>[2x]MLIKPKRLQAGDIVATVSPSWGGAGDSEIRWRYEQGVKRLEEVFGLTVVPMPNSLKGSEFIYNNPQARAEDLMTAFQDTRVKAIIANIGGQDSIRLLPYIDFNAIRENPKIFMGYADVTISHLFCHKAGLSSFYGPAILTDFAENVEMDP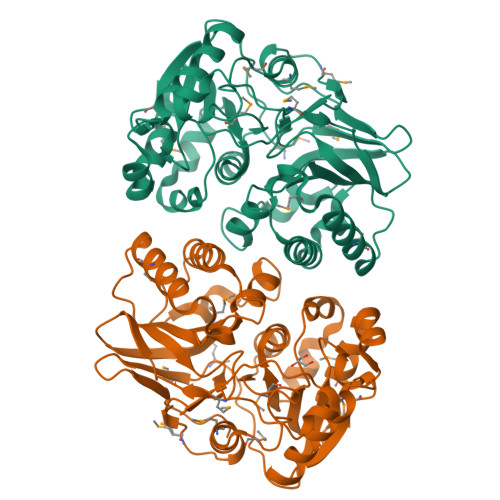YTVEMVNRTLFSNEMIGEIQPAPEWTSERLEWIEINKDTRRTMQQNNGYELLQGSTTVQGRLIGGCIEVLEFAKGTELWPEKKHWEDSILFFETSEDHPEPSYIKYWLRNYAAQGILQKAKGIIFGKPKDEMYYEEYKHEILQVMKEHNLEDLPILYNLNFGHTEPKFILPYGSMAEIDCENGSFSILESGVE>[6x]MTNLPEHQSSPTEQSSAEVKKIPTMIEGFDDISHGGLPQGRTTLVSGTSGTGKTLFAVQFLYNGITIFNEPGIFVTFEESPQDIIKNALSFGWNLQSLIDQGKLFILDASPDPDGQEVAGDFDLSALIERIQYAIRKYKATRVSIDSVTAVFQQYDAASVVRREIFRLAFRLKQLGVTTIMTTERVDEYGPVARFGVEEFVSDNVVILRNVLEGERRRRTVEILKLRGTTHMKGEYPFTINNGINIFPLGAMRLTQRSSNVRVSSGVKTLDEMCGGGFFKDSIILATGATGTGKTLLVSKFLETGCQQGERALLFAYEESRAQLSRNASSWGIDFEELERRGLLRIICAYPESAGLEDHLQIIKSEIADFKPSRVAIDSLSALARGVSNNAFRQFVIGVTGFAKQEEITGFFTNTTDQFMGSN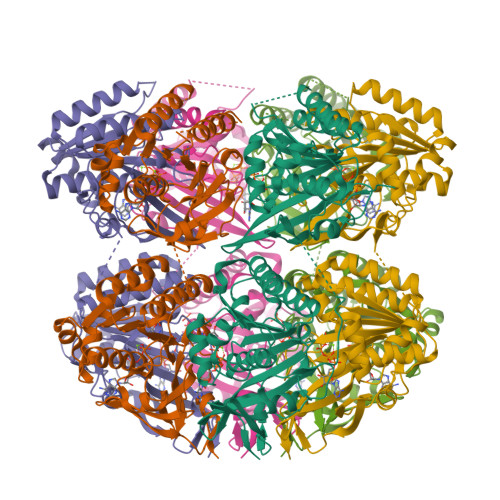SITESHISTITDTILLLQYVEIRGEMSRAINVFKMRGSWHDKGIREYVITEKGAEIRDSFRNFEGIISGTPTRISVDEKTELARIAKGMQDLESE> SDKENFWGMA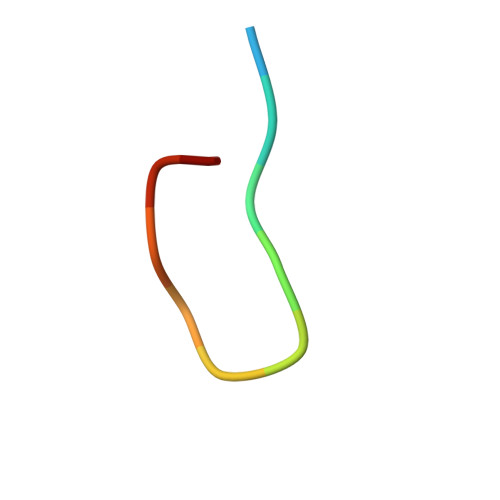VA(1~{S},3~{Z})-3-[(2~{E})-2-[(1~{S},3~{a}~{S},7~{a}~{S})-7~{a}-methyl-1-[(2~{S})-6-methyl-2-oxidanyl-hept-5-en-2-yl]-2,3,3~{a},5,6,7-hexahydro-1~{H}-inden-4-ylidene]ethylidene]-4-methylidene-cyclohexan-1-ol 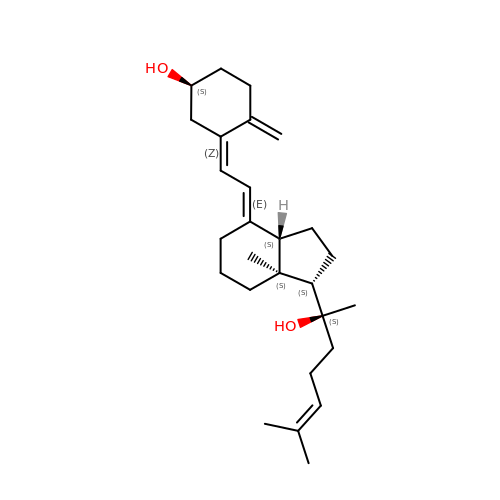| C27 H42 O2 | LZELNYSXHKHQKY-LBRHRNEPSA-N>MSVSAFNRRWAAVILEALTRHGVRHICIAPGSRSTPLTLAAAENSAFIHHTHFDERGLGHLALGLAKVSKQPVAVIVTSGTAVANLYPALIEAGLTGEKLILLTADRPPELIDCGANQAIRQPGMFASHPTHSISLPRPTQDIPARWLVSTIDHALGTLHAGGVHINCPFAEPLYGEMDDTGLSWQQRLGDWWQDDKPWLREAPRLESEKQRDWFFWRQKRGVVVAGRMSAEEGKKVALWAQTLGWPLIGDVLSQTGQPLPCADLWLGNAKATSELQQAQIVVQLGSSLTGKRLLQWQASCEPEEYWIVDDIEGRLDPAHHRGRRLIANIADWLELHPAEKRQPWCVEIPRLAEQAMQAVIARRDAFGEAQLAHRICDYLPEQGQLFVGNSLVVALIDALSQLPAGYPVYSNRGASGIDGLLSTAAGVQRASGKPTLAIVGDLSALYDLNALALLRQVSAPLVLIVVNNNGGQIFSLLPTPQSERERFYLMPQNVHFEHAAAMFELKYHRPQNWQELETAFADAWRTPTTTVIEMVVNDTDGAQTLQQL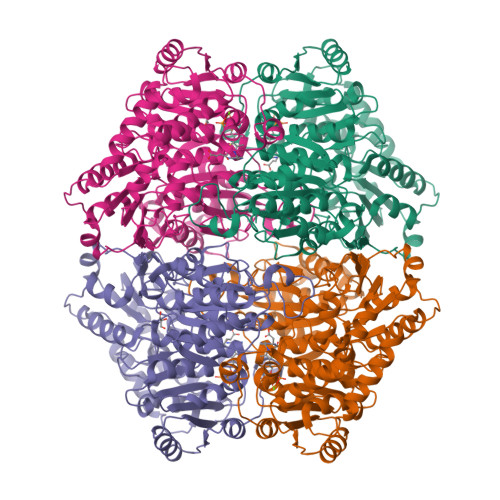LAQVSHL[8x]> MSLSNKLTLDKLDVKGKRVVMRVDFNVPMKNNQITNNQRIKAAVPSIKFCLDNGAKSVVLMSHLGRPDGVPMPDKYSLEPVAAELKSLLGKDVLFLKDCVGPEVENACANPAAGTVILLENLRFHVEEEGKGKDASGNKVKAEPAKIDAFRASLSKLGDVYVNDAFGTAHRAHSSMVGVNLPQKAGGFLMKKELNYFAKALESP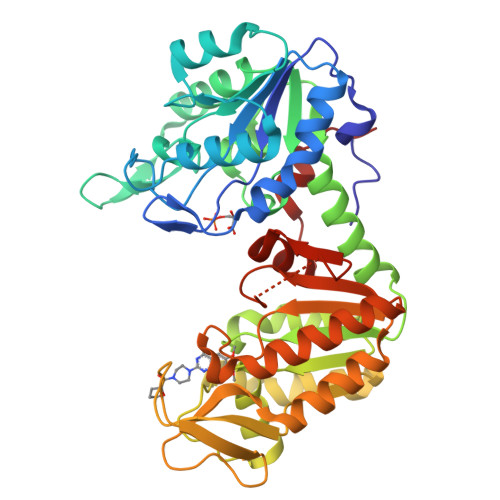ERPFLAILGGAKVADKIQLINNMLDKVNEMIIGGGMAFTFLKVLNNMEIGTSLYDEEGAKIVKDLMSKAEKNGVKITLPVDFVTADKFDENAKTGQATVASGIPAGWMGLDCGTESSKKYAEAVGRAKQIVWNGPVGVFEWEAFARGTKSLMDEVVKATSRGCITIIGGGDTATCCAKWNTEDKVSHVSTGGGASLELLEGKVLPGVDALSNV> QDNSRYTHFLTQAYDAKPQGRDDRYCESIMRRRGLT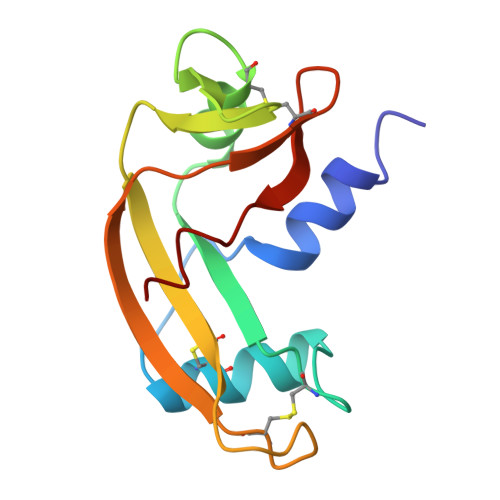SPCKDINTFIHGNKRSIKAICENKNGNPHRENLRISKSSFQVTTCKLHGGSPWPPCQYRATAGFRNVVVACENGLPVHLDQSIFRRP(2Z,4S)-5-(4-bromophenyl)-4-hydroxy-2-methylpent-2-enoic 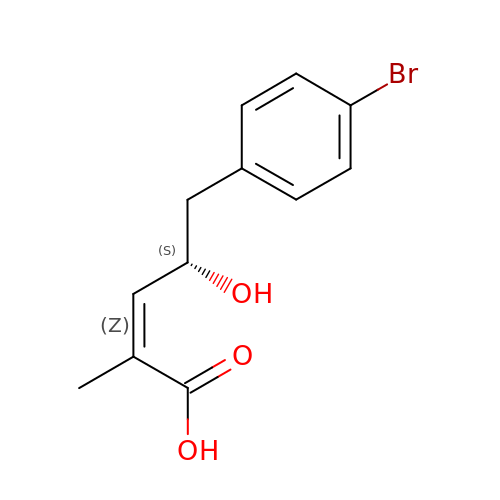acid | C12 H13 Br O3 | WYKBUUJDEZVTMI-BPOWMSRESA-N> MSRSKRDNNFYSVEIGDSTFTVLKRYQNLKPIGSGAQGIVCAAYDAILERNVAIKKLSRPFQNQTHAKRAYRELVLMKCVNHKNIIGLLNVFTPQKSLEEFQDVYIVMELMDANLCQVIQMELDHERMSYLLYQMLCGIKHLHSAGIIHRDLKPSNIVVKSDCTLKILDFGLART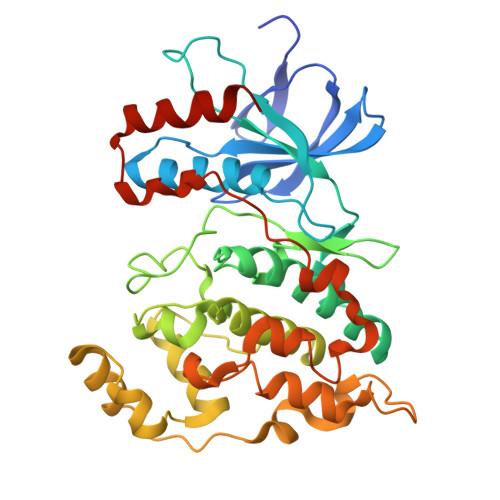AGTSFMMEPEVVTRYYRAPEVILGMGYKENVDIWSVGCIMGEMVCHKILFPGRDYIDQWNKVIEQLGTPCPAFMKKLQPTVRNYVENRPKYAGYSFEKLFPDVLFPADSEHNKLKASQARDLLSKMLVIDASKRISVDEALQHPYINVWYDPSEAEAPPPKIPDKQLDEREHTIEEWKELIYKEVMDLEHHHHHH> MQRSPLEKASVVSKLFFSWTRPILRKGYRQRLELSDIYQIPSVD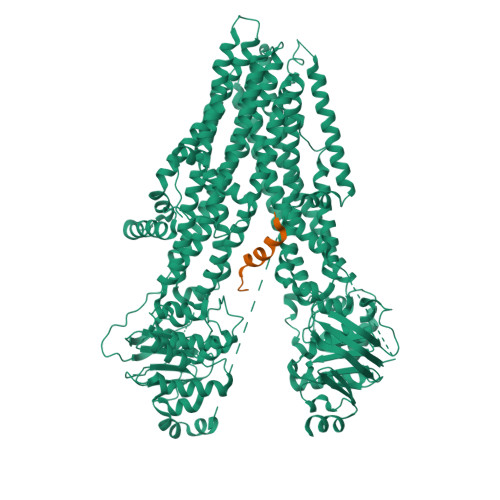SADNLSEKLEREWDRELASKKNPKLINALRRCFFWRFMFYGIFLYLGEVTKAVQPLLLGRIIASYDPDNKEERSIAIYLGIGLCLLFIVRTLLLHPAIFGLHHIGMQMRIAMFSLIYKKTLKLSSRVLDKISIGQLVSLLSNNLNKFDEGLALAHFVWIAPLQVALLMGLIWELLQASAFCGLGFLIVLALFQAGLGRMMMKYRDQRAGKISERLVITSEMIENIQSVKAYCWEEAMEKMIENLRQTELKLTRKAAYVRYFNSSAFFFSGFFVVFLSVLPYALIKGIILRKIFTTISFCIVLRMAVTRQFPWAVQTWYDSLGAINKIQDFLQKQEYKTLEYNLTTTEVVMENVTAFWEEGFGELFEKAKQNNNNRKTSNGDDSLFFSNFSLLGTPVLKDINFKIERGQLLAVAGSTGAGKTSLLMVIMGELEPSEGKIKHSGRISFCSQFSWIMPGTIKENIIFGVSYDEYRYRSVIKACQLEEDISKFAEKDNIVLGEGGITLSGGQRARISLARAVYKDADLYLLDSPFGYLDVLTEKEIFESCVCKLMANKTRILVTSKMEHLKKADKILILHEGSSYFYGTFSELQNLQPDFSSKLMGCDSFDQFSAERRNSILTETLHRFSLEGDAPVSWTETKKQSFKQTGEFGEKRKNSILNPINSIRKFSIVQKTPLQMNGIEEDSDEPLERRLSLVPDSEQGEAILPRISVISTGPTLQARRRQSVLNLMTHSVNQGQNIHRKTTASTRKVSLAPQANLTELDIYSRRLSQETGLEISEEINEEDLKECFFDDMESIPAVTTWNTYLRYITVHKSLIFVLIWCLVIFLAEVAASLVVLWLLGNTPLQDKGNSTHSRNNSYAVIITSTSSYYVFYIYVGVADTLLAMGFFRGLPLVHTLITVSKILHHKMLHSVLQAPMSTLNTLKAGGILNRFSKDIAILDDLLPLTIFDFIQLLLIVIGAIAVVAVLQPYIFVATVPVIVAFIMLRAYFLQTSQQLKQLESEGRSPIFTHLVTSLKGLWTLRAFGRQPYFETLFHKALNLHTANWFLYLSTLRWFQMRIEMIFVIFFIAVTFISILTTGEGEGRVGIILTLAMNIMSTLQWAVNSSIDVDSLMRSVSRVFKFIDMPTEGKPTKSTKPYKNGQLSKVMIIENSHVKKDDIWPSGGQMTVKDLTAKYTEGGNAILENISFSISPGQRVGLLGRTGSGKSTLLSAFLRLLNTEGEIQIDGVSWDSITLQQWRKAFGVIPQKVFIFSGTFRKNLDPYEQWSDQEIWKVADEVGLRSVIEQFPGKLDFVLVDGGCVLSHGHKQLMCLARSVLSKAKILLLDEPSAHLDPVTYQIIRRTLKQAFADCTVILCEHRIEAMLECQQFLVIEENKVRQYDSIQKLLNERSLFRQAISPSDRVKLFPHRNSSKCKSKPQIAALKEETEEEVQDTRLSNSLEVLFQ> MDEGAKQTDIQSYVADMQPGWNLGNTFDAVGDDETAWGNPRVTR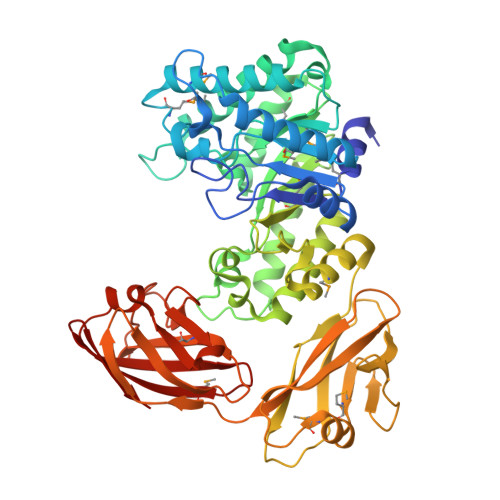ELIKTIADEGYKSIRIPVTWENQMGNAPDYTINEDFFSRVEQVIDWALEEDLYVMLNLHHDSWLWIYNMEHNYDEVMAKYTALWEQLSERFQGHSHKLMFESVNEPRFTRDWGEIQENHHAFLEELNTAFYHIVRESGGSNTERPLVLPTLETATSQDLLNRLHQTMKDLNDPNLIATVHYYGFWPFSVNVAGYTRFEEETQQDIIDTFNRVHNTFTANGIPVVLGEFGLLGFDTSTDVIQQGEKLKFFEFLIHHLNERDVTHMLWDNGQHLNRETYSWYDQEFHNMLKASWEGRSATAESNLIHVRDGEPIRDQDIQLHLHGNELTGLQVDGDSLALGEDYELAGDVLTMKADALTALMTPGELGTNAVITAQFNSGADWHFQLQNVDEPTLENTEGSTSNFAIPAHFNGDSVATMEAVYANGEFAGPQNWTSFKEFGYTFSPVYDKGEIVITDAFFNEVRDDDIHLTFHFWSGEMVEYTLSKNGNHVQGRR>[2x]GPQPPADEQPEPRTRRRAYLWCKEFLPGAWRGLREDEFHISVIRGG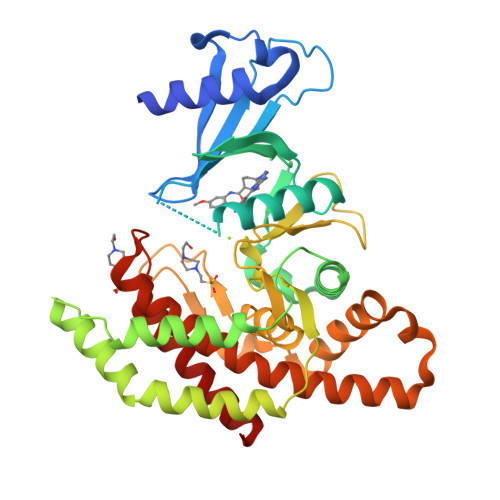LSNMLFQCSLPDTTATLGDEPRKVLLRLYGAILQMRSCNKEGSEQAQKENEFQGAEAMVLESVMFAILAERSLGPKLYGIFPQGRLEQFIPSRRLDTEELSLPDISAEIAEKMATFHGMKMPFNKEPKWLFGTMEKYLKEVLRIKFTEESRIKKLHKLLSYNLPLELENLRSLLESTPSPVVFCHNDCQEGNILLLEGRENSEKQKLMLIDFEYSSYNYRGFDIGNHFCEWMYDYSYEKYPFFRANIRKYPTKKQQLHFISSYLPAFQNDFENLSTEEKSIIKEEMLLEVNRFALASHFLWGLWSIVQAKISSIEFGYMDYAQARFDAYFHQKRKLGV>[2x]SMPFPEGKVLDDMEGNQWVLGKKIGSGGFGLIYLAFPTNKPEKDARHVVKVEYQENGPLFSELKFYQRVAKKDCIKKWIERKQLDYLGIPLFYGSGLTEFKGRSYRFMVMERLGIDLQKISGQNGTFKKSTVLQLGIRMLDVLEYIHENEYVHGDIKAANLLLGYKNPDQVYLADYGLSYRYCPNGNHKQYQENPRKGHNGTIEFTSLDAHKGVALSRRSD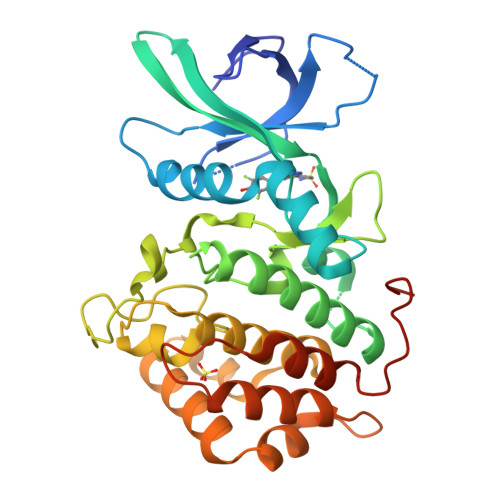VEILGYCMLRWLCGKLPWEQNLKDPVAVQTAKTNLLDELPQSVLKWAPSGSSCCEIAQFLVCAHSLAYDEKPNYQALKKILNPHGIPLGPLDFSTKGQSINVH> MKQLSTDAERELANIWATVLDIPIGTISASDNFFFRGGHSIDAMKASALGRAAGMSFGVADIFDHPV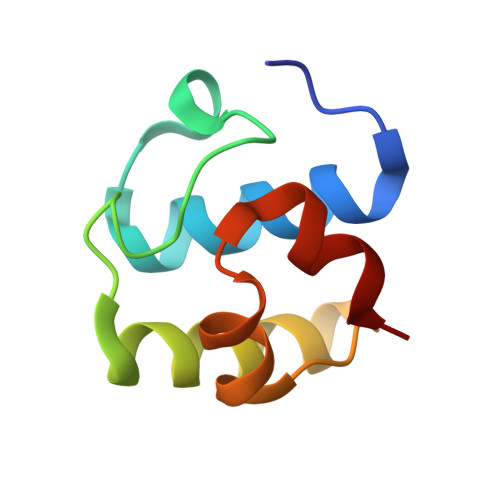LSELASVAVA> IVGGRKARPRQFPFLASIQNQGRHFCGGALIHARFVMTAASCFQSQNPGVSTVVLGAYDLRRRERQSRQTFSISSMSENGYDPQQNLNDLMLLQLDREANLTSSVTILPLPLQNATVEAGTRCQVAGWGSQRSGGRLSRFPRFVNVTVTPEDQCR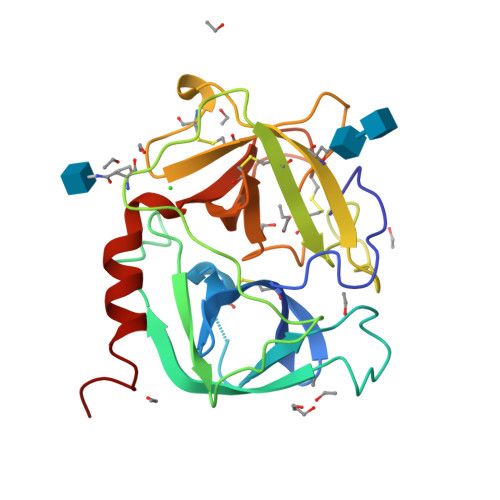PNNVCTGVLTRRGGICNGDGGTPLVCEGLAHGVASFSLGPCGRGPDFFTRVALFRDWIDGVLNNPGPGPA>GASGAPKLQPFTFPKTLHEGQTVKAICTPTEGERPLQFQWLKDGHPLMKRPLVDIKTFEDYSLLKVSSVGEKDIGNYTCIVRNHHGSDQFTTSLTIPVA[2x]

Recently, a shortened Dscam (sDscam) gene family with tandemly arrayed 5′ cassettes in Chelicerata species has been identified, which encodes ∼50–100 isoforms. Chelicerata sDscams could be classified into two subfamilies, sDscamα and sDscamβ, containing one and two variable Ig domains, respectively. Crystal structures and cell aggregation assays demonstrated that both α and β subfamilies of sDscam used Ig1 for the isoform-specific trans recognition in a hand-in-hand manner. Furthermore, the cis interactions were established by the three FNIII domains of sDscam, which assemble into a cross fold with a kink between FNIII2 and FNIII3.

We also determined the crystal structures of sDscam Ig1 from another chelicerate species Limulus polyphemus (isoforms α7 and β3v7) to provide insights into the conservation of sDscam trans recognition within Chelicerata. These crystal structures of Ig fragments were determined at 1.3–3.1 Å resolutions. The crystal structures of sDscam Ig1 from both M. martensii and L. polyphemus revealed a common assembly of antiparallel homodimer for both α and β subfamilies of sDscam. In addition, all these Ig1 homodimers resemble each other well with root mean square deviation (RMSD) values of 1.0–1.6 Å, indicating a shared mechanism of sDscam trans recognition within Chelicerata. Similarly, sDscam Ig1 also employs the ABED face to form an antiparallel homodimer. However, among the seven Ig1 structures reported here, the complementary electrostatic potential surface pattern (negative in one end, neutral in the middle, and positive in the other end) has been only observed in the three β isoforms, but not in any one of the four α isoforms. Electrostatic and shape complementarity had been observed in all Ig1 dimer interfaces.Some bacteria express a binary toxin translocation system, consisting of an enzymatic subunit and translocation pore, that delivers enzymes into host cells through endocytosis. The B-components of the C. perfringens, C. difficile, and C. spiroforme systems bind to the host cell’s lipolysis-stimulated lipoprotein receptor (LSR), after which the A–B complex is internalized by endocytosis. Then, the A-component is translocated via the B-component pore across the endosomal membrane into the cytosol, assisted by host-cell chaperones, including Hsp90 and Hsp70. In the cytosol, the A-component covalently transfers an ADP-ribose to actin, causing F-actin depolymerization, cell rounding, and eventually cell death.

Here, we report two cryo-EM structures of the CDTa-bound CDTb-pore, long and short, at 2.64- and 2.56-Å resolution, respectively. We solved two structures of CDTa-bound CDTb-pores: one with a long stem and the other with a short stem. The former contained one entire β-barrel stem; however, the final map calculation showed that the tip of this stem (residues 337–358) had very weak density; therefore, we modeled the structure with a partial β-barrel stem, excluding residues 337–358. Thus, both the long and short structures have partial β-barrel stems, lacking β-barrel tip residues 337–358 and 332–363, respectively. The most striking difference between the structures was that D4II (receptor-binding domain II) was observed in the long, but not in the short complex. Between the long and the short structures, the definitive difference is that D4II is clearly visible in the long form. That is, after stem formation, D4II is stably fixed around the stem. Domain 4 is the receptor-binding domain at the outermost region of the pore, with two sub-domains, D4I (T617–L741) and D4II (T757–D876), joined through a linker (N742–P756), as seen in the long-form. However, the two overall structures were similar, including a 1:1 binding ratio of CDTa:CDTb-pore. In both the long and short complexes, CDTa was bound to the cis-side of the CDTb-pore through its N-terminal domain.

>[7x]NNNFFDPKLMSDWEDEDLDTDNDNIPDSYERNGYTIKDLIAVKWEDSFAEQGYKKYVSNYLESNTAGDPYTDYEKASGSFDKAIKTEARDPLVAAYPIVGVGMEKLIISTNEHASTDQGKTVSRATTNSKTESNTAGVSVNVGYQNGFTANVTTNYSHTTDNSTAVQDSNGESWNTGLSINKGESAYINANVRYYNTGTAPMYKVTPTTNLVLDGDTLSTIKAQENQIGNNLSPGDTYPKKGLSPLALNTMDQFSSRLIPINYDQLKKLDAGKQIKLETTQVSGNFGTKNSSGQIVTEGNSWSDYISQIDSISASIILDTENESYERRVTAKNLQDPEDKTPELTIGEAIEKAFGATKKDGLLYFNDIPIDESCVELIFDDNTANKIKDSLKTLSDKKIYNVKLERGMNILIKTPTYFTNFDDYNNYPSTWSNVNTTNQDGLQGSANKLNGETKIKIPMSELKPYKRYVFSGYSKDPLTSNSIIVKIKAKEEKTDYLVPEQGYTKFSYEFETTEKDSSNIEITLIGSGTTYLDNLSITELNSTPEILDEPEVKIPTDQEIMDAHKIYFADLNFNPSTGNTYINGMYFAPTQTNKEALDYIQKYRVEATLQYSGFKDIGTKDKEMRNYLGDPNQPKTNYVNLRSYFTGGENIMTYKKLRIYAITPDDRELLVLSVD;> APIERPEDFLKDKEKAKEWERKEAERIEQKLERSEKEALESYKKDSVEISKYSQTRNYFYDYQIEANSREKEYKELRNAISKNKIDKPMYVYYFESPEKFAFNKVIRTENQNEISLEKFNEFKETIQNKLFKQDGFKDISLYEPGKGDEKPTPLLMHLKLPRNTGMLPYTNTNNVSTLIEQGYSIKIDKIVRIVIDGKHYIKAEASVVSSLDFKDDVSKGDSWGKANYNDWSNKLTPNELADVNDYMRGGYTAINNYLISNGPVNNPNPELDSKITNIENALKREPIPTNLTVYRRSGPQEFGLTLTSPEYDFNKLENIDAFKSKWEGQALSYPNFISTSIGSVNMSAFAKRKIVLRITIPKGSPGAYLSAIPGYAGEYEVLLNHGSKFKINKIDSYKDGTITKLIVDATLIPENLYFQGLEHHHHHH>LATTSDHDFSYLSFAYDATDLELEGSYDYVIVGGGTSGCPLAATLSEKYKVLVLERGSLPTAYPNVLTADGFVYNLQQEDDGKTPVERFVSEDGIDNVRGRVLGGTSIINAGVYARANTSIYSASGVDWDMDLVNQTYEWVEDTIVYKPNSQSWQSVTKTAFLEAGVHPNHGFSLDHEEGTRITGSTFDNKGTRHAADELLNKGNSNNLRVGVHASVEKIIFSNAPGLTATGVIYRDSNGTPHQAFVRSKGEVIVSAGTIGTPQLLLLSGVGPESYLSSLNIPVVLSHPYVGQFLHDNPRNFINILPPNPIEPTIVTVLGISNDFYQC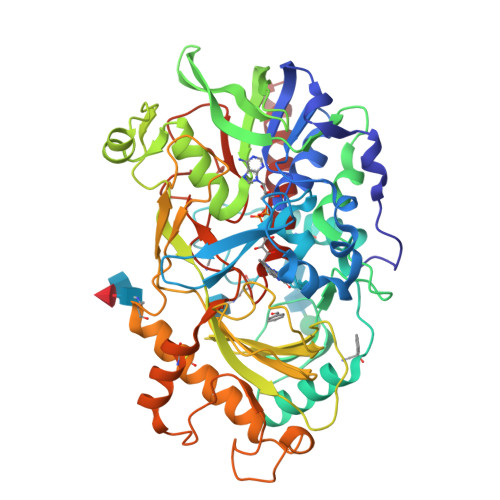SFSSLPFTTPPFGFFPSSSYPLPNSTFAHFASKVAGPLSYGSLTLKSSSNVRVSPNVKFNYYSNLTDLSHCVSGMKKIGELLSTDALKPYKVEDLPGVEGFNILGIPLPKDQTDDAAFETFCRESVASYWHYHGGCLVGKVLDGDFRVTGINALRVVDGSTFPYTPASHPQGFYLMLGRYVGIKILQERSASD[2x]>[6x]SDEAVGDLKQALPCVAESPTVHVEVHQRGSSTAKKEDINLSVRKLLNRHNIVFGDYTWTEFDEPFLTRNVQSVSIIDTELKVKDSQPIDLSACTVALHIFQLNEDGPSSENLEEETENIIAANHWVLPAAEFHGLWDSLVYDVEVKSHLLDYVMTTLLFSDKNVNSNLITWNRVVLLHGPPGTGKTSLCKALAQKLTIRLSSRYRYGQLIEINSHSLFSKWFSESGKLVTKMFQKIQDLIDDKDALVFVLIDQVESLTAARNACRAGTEPSDAIRVVNAVLTQIDQIKRHSNVVILTTSNITEKIDVAFVDRADIKQYIGPPSAAAIFKIYLSCLEELMKCQIIYPRQQLLTLRELEMIGFIENNVSKLSLLLNDISRKSEGLSGRVLRKLP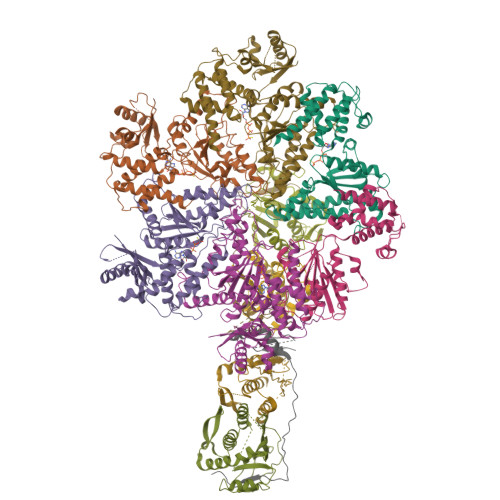FLAHALYVQAPTVTIEGFLQALSLAVDKQFEERKKLAAYI;>STTLTRQDLNFGQVVADVLCEFLEVAVHLILYVREVYPVGIFQKRKKYNVPVQMSCHPELNQYIQDTLHCVKPLLEKNDVEKVVVVILDKEHRPVEKFVFEITQPPLLSISSDSLLSHVEQLLRAFILKISVCDAVLDHNPPGCTFTVLVHTREAATRNMEKIQVIKDFPWILADEQDVHMHDPRLIPLKTMTSDILKMQLYVEERAHKGS[4x];>[2x]MSQVHIFWGAPIAPLKGSGSGSGSGSGSGSGSTTEVILHYRPCESDPTQLPKIAEKAIQDFPTRPLSRFIPWFPYDGSKLPLRPKRSPPASREEIMATL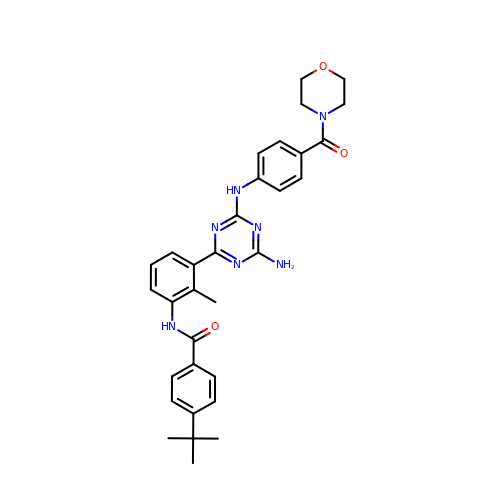N-[3-(4-amino-6-{[4-(morpholine-4-carbonyl)phenyl]amino}-1,3,5-triazin-2-yl)-2-methylphenyl]-4-tert-butylbenzamide | C32 H35 N7 O3 | BRQYZNVVGDQNTM-UHFFFAOYSA-N3'-DEOXYURIDINE-5'-MONOPHOSPHATE 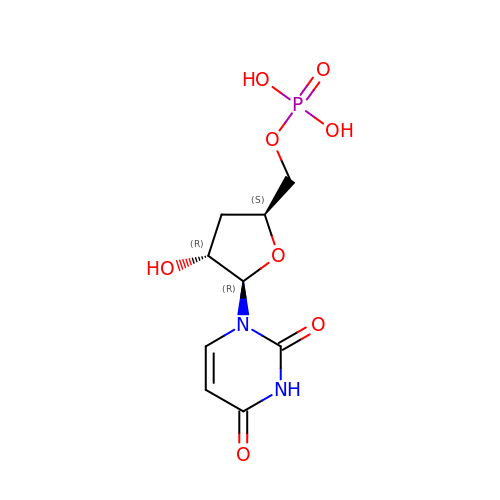| C9 H13 N2 O8 P | SEOHEWZQAGEAGZ-SHYZEUOFSA-N>[10x]DLLSWFKGNDRPPAPAGKALEFSKPAAWQNNLPLT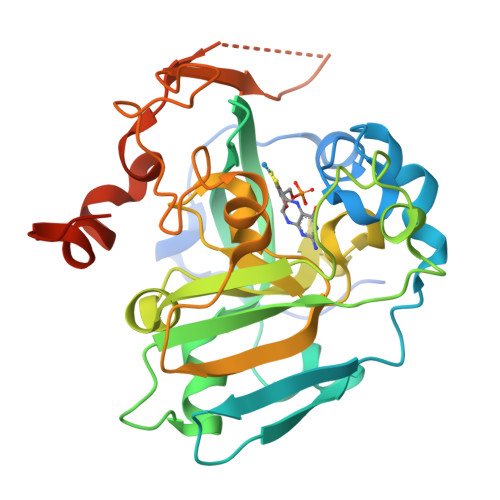PADKVSGYNNFYEFGLDKADPAANAGSLKTDPWTLKISGEVAKPLTLDHDDLTRRFPLEERIYRMRCVEAWSMVVPWIGFPLHKLLALAEPTSNAKYVAFETIYAPEQMPGQQDRFIGGGLKYPYVEGLRLDEAMHPLTLMTVGVYGKALPPQNGAPVRLIVPWKYGFKGIKSIVSIKLTRERPPTTWNLAAPDEYGFYANVNPYVDHPRWSQATERFIGSGGILDVQRQPTLLFNGYADQVASLYRGLDLRENFLEHHHHHH>[4x]GQSRERLVKWLQDAYAMEKEAETMMAAMASRIEH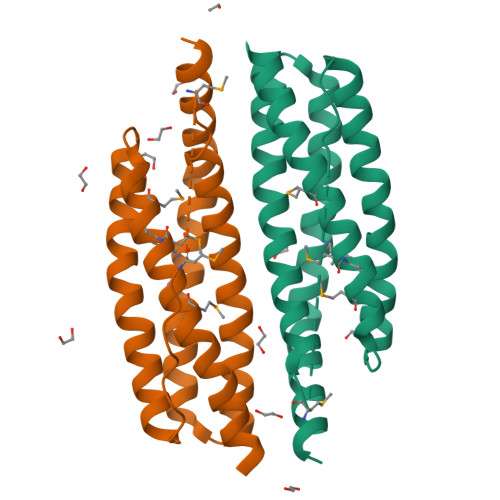YPELKRRIEQHVEETQQQSAGVQRCLELLNGSIPTAKGMLSSVLASMHAAGNSMMTDEVTKGVGISYAFEHLEIASYRALVVAARSAGEQEVAQICEDILQQEIEMAEWLIEHQEAIVVAFLEREQLEGVGS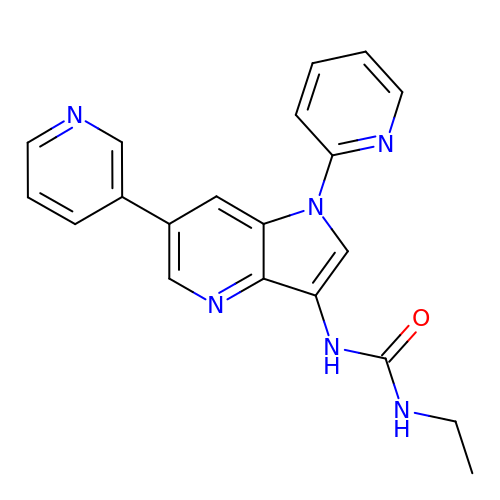1-ethyl-3-[1-(pyridin-2-yl)-6-(pyridin-3-yl)-1H-pyrrolo[3,2-b]pyridin-3-yl]urea | C20 H18 N6 O | FRDSIJNIQUPVHU-UHFFFAOYSA-N> SHMMRNRSVRNIVWDIGEKLSDYEKVKEIVNNEKNYINFEGNFLNPFNELSLSHGIPALCVLYGELNEQYPEQGWDVIGHEYMKRMGEYIEEKGITSLSMFSGVSGIGLSAVCLSNNRSRYGNFISSMNSFIEENIPGFIEILRNKESLNMSDYDVIEGVCGIANYCMLFPNNEEMKQALRLIVGYIIELCKDKTINGLVLPGWYISAENQFSKVDQKLWPEGCFNIGLSHGVPGMLLVLCNSTKCGIHLEDQDDSINKLVDFLIKFHISNDKENYWGSHISLEEYREGKVNSTNSRDAWCYGTPGAAYSVLIAGKYLNNMEYIDEAVNAMKGAINRLRDIYSPTFCHGFSGIAYISNRFYEVTKQQDFKKAAIDLTDKILELYDEKAPFGFYN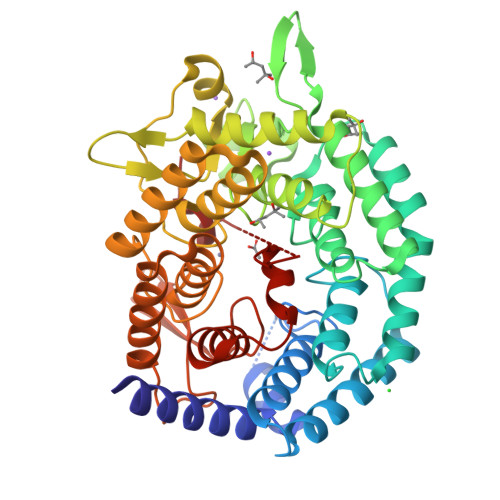MEKSEEGMDYLDYIGIIDGVTGIILTLLAIENGKKTPWDCAFSLQEVAAAHHAAA>MRRSHTIGVVTTGLSFYGPSQILVGIERAAREHGYSLLLATVHEDPDEVEEAINTLRERRVDGIIIVAPHNSEEEAQLAQEAGVPPVVFLSAQPPGVPTVSVDQYAGARLATEHLLDLGHRRIALITGPQDWLEARERLQGWREALAEAGLPPPAVLQGDWSAASGYEAARQLLEQPDFTAIFAANDQMALGVLRALHERGLRVPDDVSVVGFDDIPESAYFHPPLTTVRQDFEELGRQAVEQLLEMIEGEEPPPPAVLPPELIVRESTAP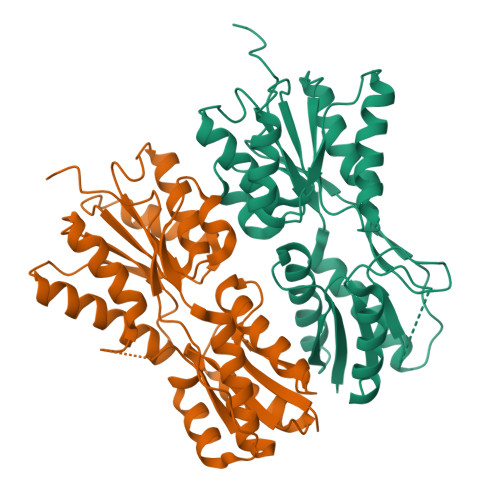PENLYFQGL[4x]>[2x]GNKYIQQTKPLTLERTINLYPLTNYTFGTKEPLYEKDSSVAARFQRMREEFDKIGMRRTVEGVLIVHEHRLPHVLLLQLGTTFFKLPGGELNPGEDEVEGLKRLMTEILGRQDGVLQDWVIDDCIGNWWRPNFEPPQYPYIPAHITKPKEHKKLFLVQLQEKALFAVPKNYKLVAAPLFELYDNAPGYGPIISSLPQLLSRFNFIYN;>[2x]DVGEEFNQE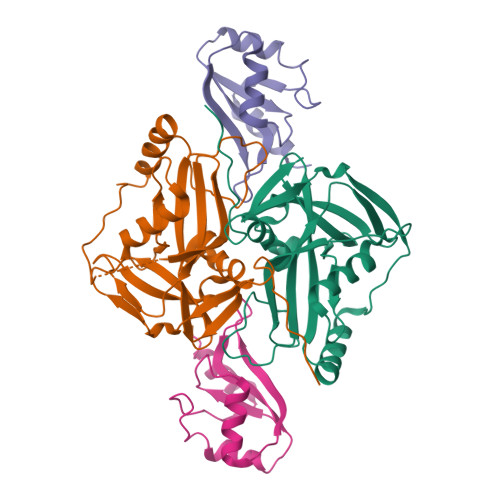AEYGGHDQIDLYDDVISPSANNGDAPEDRDYMDTLPPTVGDDVGKGAAPNVVYTYTGKRIALYIGNLTWWTTDEDLTEAVHSLGVNDILEIKFFENRANGQSKGFALVGVGSEASSKKLMDLLPKRELHGQNPVVTPVNKQFLSQFEMQSRKTTQSGQMSGEGKAGPPGGSSRAAFPQGGRGRGRFPGAVPGGDRFPGPAGPGGPPPPFPAGQTHHHHHH>GPLGSSASEGMKFKFHSGEKVLCFEPDPTKARVLYDAKIVDVIVGKDEKGRKIPEYLIHFNGWNRSWDRWAAEDHVLRDTDENRRLQRKLARKA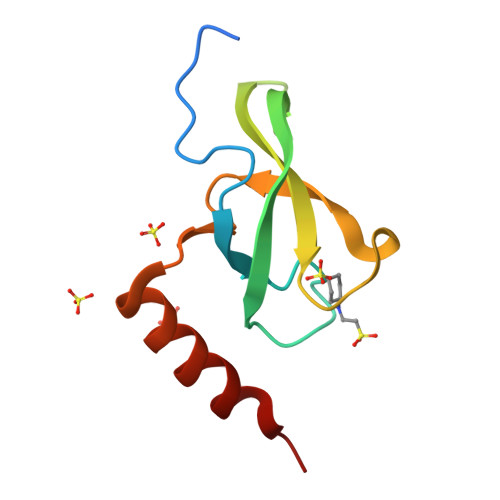VAR[5x]> XATSRYEPVAEIGVGAYGTVYKARDPHSGHFVALKSVRVPNGGGGGGGLPISTVREVALLRRLEAFEHPNVVRLMDVCATSRTDREIKVTLVFEHVDQDLRTYLDKAPPPGLPAETIKDLMRQFLRGLDFLHANCIVHRDLKPENILVTSGGTVKLADFGLARIYSYQMALTPVVVTLWYRAPEVLLQSTYATPVDMWSVGCIFAEMFRRKPLFCGNSEADQLGKIFDLIGLPPEDDWPRDVSLPRGAFPPRGPRPVQSVVPEMEESGAQLLLEMLTFNPHKRISAFRALQHSYLHKDEGNPEEGHHHHHH;> MELLCCEGTRHAPRAGPDPRLLGDQRVLQSLLRLEERYVPRASYFQCVQREIKPHMRKMLAYWMLEVCEEQRCEEEVFPLAMNYLDRYLSCVPTRKAQLQLLGAVCMLLASKLRETTPLTIEKLCIYTDHAVSPRQLRDWEVLVLGKLKWDLAAVIAHDFLAFILHRLSLPRDRQALVKKHAQTFLALCATDYTFAMYPPSMIATGSIG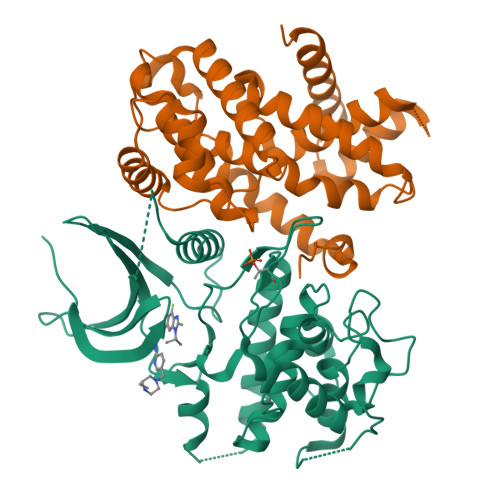AAVQGLGACSMSGDELTELLAGITGTEVDCLRACQEQIEAALRESLREAS> SNADAESLFREALSNKVDELAHFLLRKYRAKELVTKAEMLERVIKNYKRCFPVIFGKASESLKMIFGIDVKEVDPTSNTYTLVTCLGLSYDGLLGNNQIFPKTGLLIIVLGTIAMEGDSASEEE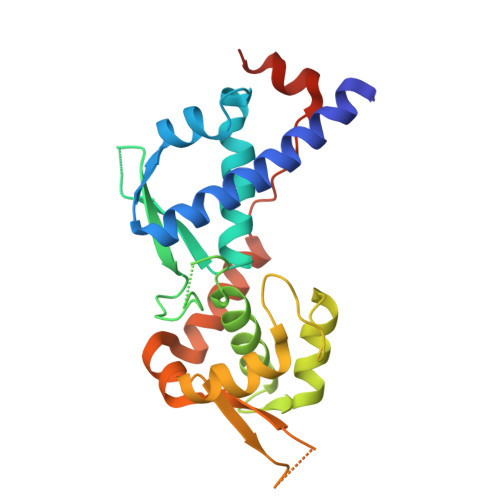IWEELGVMGVYDGREHTVYGEPRKLLTQDWVQENYLEYRQVPGSNPARYEFLWGPRALAETSYVKVLEHVVRVNARVRIAYPSLREAALLEEEEGV>[2x]SNADIMGFVFNTRRTLFKDKRVRQALSILFDFEWVNHHLFNNIYTRTEGYWDGSILSSIGKPASEEEKALLAPYPDAVLPEVMDGSWRISK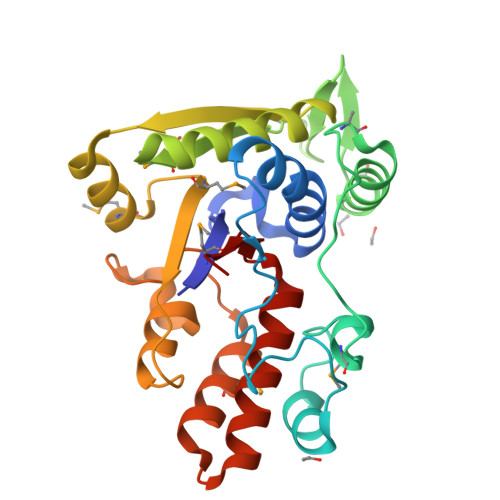TDGSGMDRLNAQKAWKLLQEAGFTKKNNRLIAPNGLPFQFEIMTQSLEEEKVALAFQSNLSRLGIHAEIRTVDDSQYQNRLGMFNYDMIIGKLKNSLSPGNEQINRWSSASRNLKGSFNFSGASDPAIDAMITAILDAHSQVDFIAAVRALDRILISGSYYIPLYHLS>MHHHH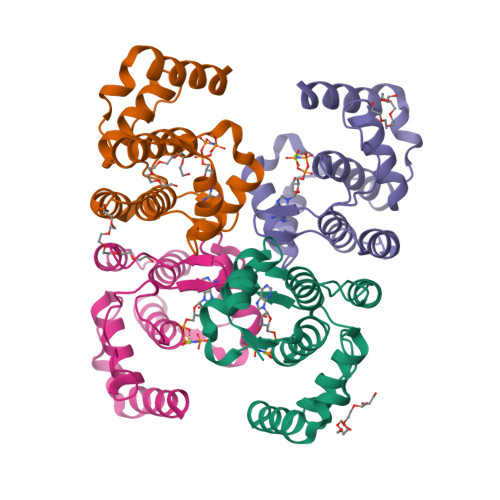HHMKSIDEQSLHNARRLFESGDIDRIEVGTTAGLQQIHRYLFGGLYDFAGQIREDNISKGGFRFANAMYLKEALVKIEQMPERTFEEIIAKYVEMNIAHPFLEGNGRSTRIWLDLVLKKNLKKVVNWQNVSKTLYLQAMERSPVNDLELRFLLKDNLTD[4x]>EVASYCDRVVAAVSSWMSTVKSTTEVSWNKLSFCDVLLKIITFGIYSPHETLAEKYSEKKLMDSFSPSLSQDKMDGEFAHANIDGISIRLCLNKGICSVFYLDGDKIQSTQLSSKEYNNLLSSLPPKQFNLGKVHTITAPVSGNFKTHKPAPEVIETAINCCTSIIPNDDYFPVKDTDFNSVWHDIYRDIRASDSNSTKIYFNNIEIPLKLIADLINELGINEFIDSKKELQMLSYNQLNKIINSNFPQQDLCFQTEKLLFTSLFQDPAFISALTSAFWQSLHITSSSVEHIYAQIMSENIENRLNFMPEQ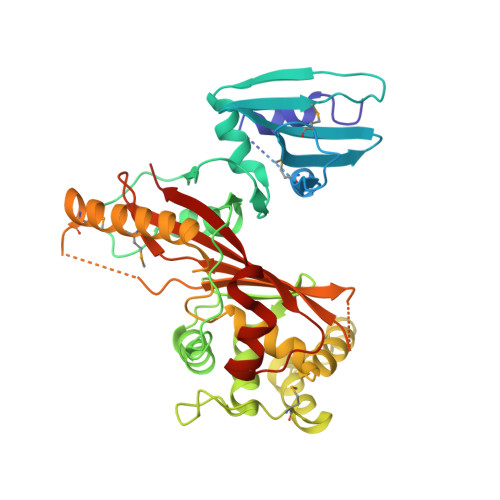RVINNCGHIIKINAVVPKNDTAISASGGRAYEVSSSILPSHITCNGVGINKIETSYLVHAGTLPSSEGLRNAIPPESRQVSFAIISPDV[2x]> MV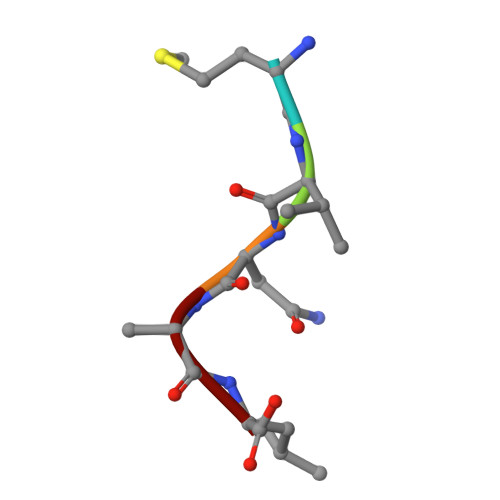NAL>[2x]MEFRSLGRSGLSVSEIVYGNLLYPQDDTPDEVVLSSIRAALDAGVTTFDTADVYGMFRSESLLGRALAGTPREELVLCTKVGMPTGFGPNGRGLSRKHVMESVDGSLRRLRVDHIDVYTAHRYDPATPLEELMWTFSDLVRAGK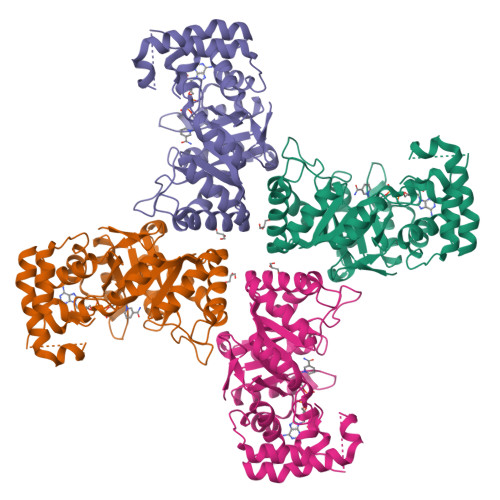ILYVGMSEWPVERIAEAAGIGARLGVPVICHMPRYSMLWRAPEAEVIPACRDLGIGQICYFTLEQGVLTGKYAPGAPPPAGSRATAPKGGRAPLMRRWLDDDKVLGRVERLRPLAEEAGLTTAQLALAWVLQNPGVSGAVIGSFNAEQVLANAESAGVRLETDLLVRIDEVLGDSVVHDEELEHHHHHH>MVNKTEKTSDLMFERFKRNVSEIV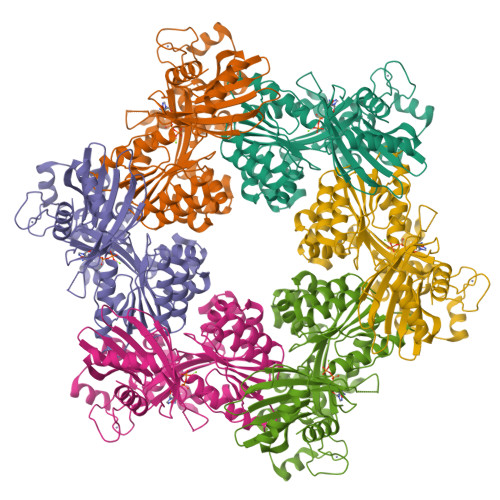TGDGGELELTVEQRKYFLIFKNGDFLVSSCHMKHHLVQMLREIATRKGYPNLTIYEVNLKDIRLLYEASLKTVQNNGQDLLPVEKRASMLLFECAEMRVSDLHIKVYDAEADIYIRKDGDMELLRQIESNTAHSILASLYNNADDSDATYKINAYQAARIVASKSRLALPPVIQAVRLQFNPLGQGGRYLIARFLYTDKSEKQKEMDPTRFGFHHSHAESFSRMRNLPIGINIISGPTGSGKSTTLKNLLELLYIEKKKKVNIISIEDPPEYEIDGTAQLPITNVETEAQRGEEYRKAITAALRSDPDIIMPGEARDAEVINLLFTAAMTGHQVWTSLHANNALAIFDRLKDQGVDEFKLTDPELITGLVAQRLVRKLCAQCSITLTEYIASGGGISDTDRKIISGHETSVRFPNPRAKKCCRDGYNGRTILAEVIEPDSKLLRLVAEGKREDAQHYWLTSLHGMALKEHAWLKIISGEICVMDAVNKISGIDNITEERKKYLFSRDNEI[6x]> PLREGLGPLQIWQTDFTLEPRMAPRSWLAVTVDTASSAIVVTQHGRVTSVAAQHHWATAIAVLGRPKAIKTDNGSCFTSKSTREWLARWGIAHTTGIPGNSQGQAMVERANRLLKDKIRVLAEGDGFMKRIPTSKQGELLAKAMYAL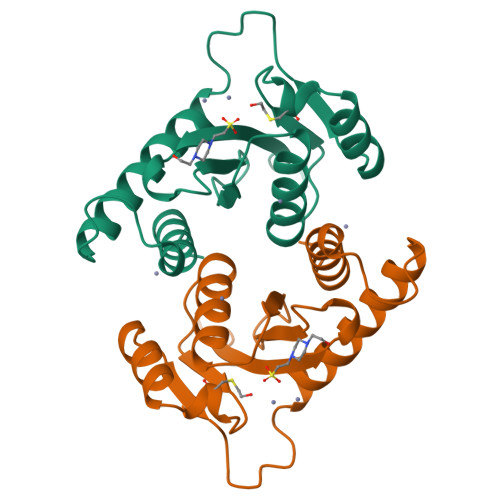NHFNL>[4x]EEGQKVDHCARHGEKLLLFCQEDSKVICWLCERSQEHRGHHTFLMEEVAQEYHVKLQTALEMLRQKQQEAETERNQVAKRVPKAPP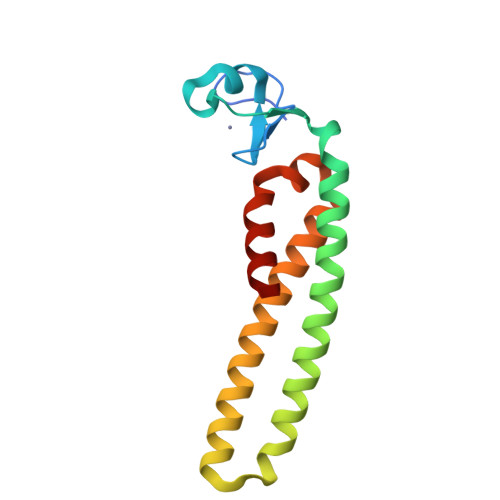EEKEALIARGKALGEQTQYMRELISELEHRLQGSMMDLLQGVDGIIKRIENMTLK ADENOSINE-5'-DIPHOSPHATE-GLUCOSE | C16 H25 N5 O15 P2 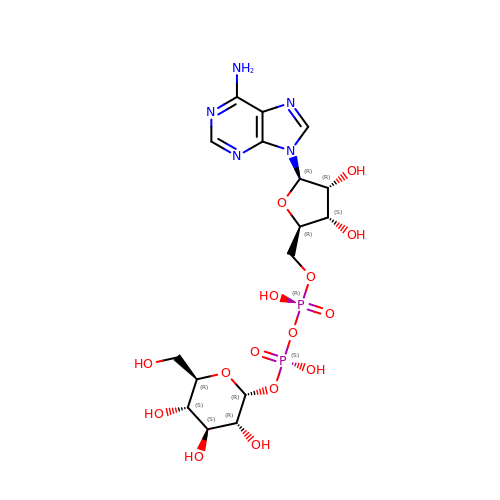| WFPZSXYXPSUOPY-ROYWQJLOSA-N> IADRVRTSWTYRHSRYSGGVRFSLPRFMVTKRTYLSTKFRRPSTVTKWGNPQYTLPSNVQREMQENSAEGDTDQATSEELGGRTGKKE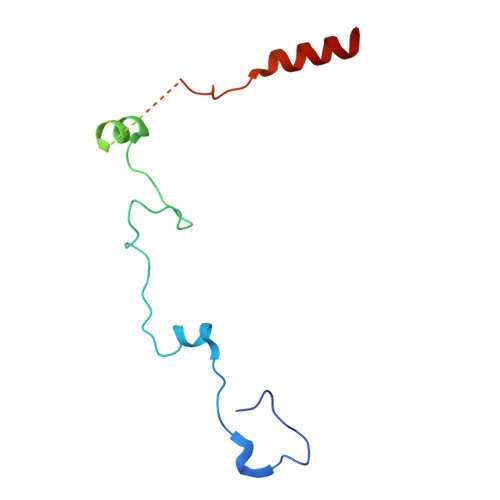LGRNGKSAGKTKKAADTAAQEVQHTPKYCDMLFLHQEDQQSRRR>[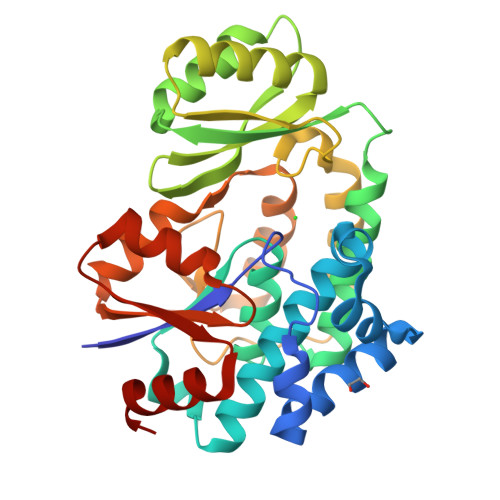2x]GPGSMGAAFTFPGQGSQLIGMGKVLTEQFVAARMVFEEVDDALSEKLSDIIFEGPADVLTLTANAQPALMAVSMAVIRVMEQLGLNVEKKVKFVAGHSLGEYSALCAAGTFSLTDTARLLRIRGNAMQAAVAVGEGSMAALIGLDEKDVEEICEIVAEEGLCQIANDNGGGQIVISGEAKAVETAVEVASQKGAKRAVLLPVSAPFHSALMQPAANAMKNALLTVNKTAPIVPLIANVSVIPESDPERIVSLLVQQVTGRVRWRETIEWISANGVNTLFEIGSGKVLTGLARRINKDIKALTVGTAEEIEAALRVLGV>[2x]AAPTTPGAGAPCAACKFLRRKCLPGCVFAPYFPPEEPQKFANVHKVFGASNVTKLLNELPPHQREDAVSSLAYEAEARVKDPVYGCVGAISVLQRQVH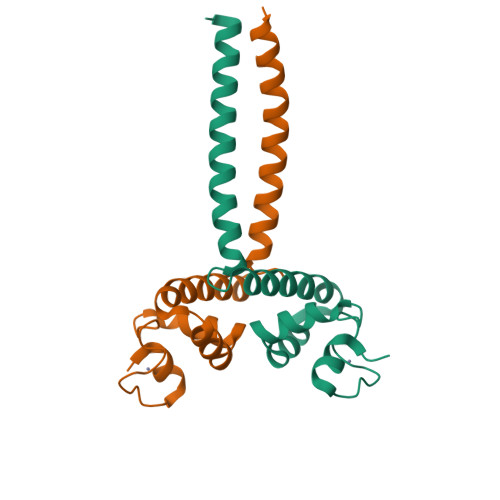RLQKELDAAHTELLRYACGELGGIPTALPVVTA>[4x]MFPDGFVWGTSTAAYQIEGAVAEDGRTPSIWDTFSRTKGKVVNGDTGDVACDHYHRWEEDLDLLAELGVQAYRFSVAWPRIHPDVTGPANQ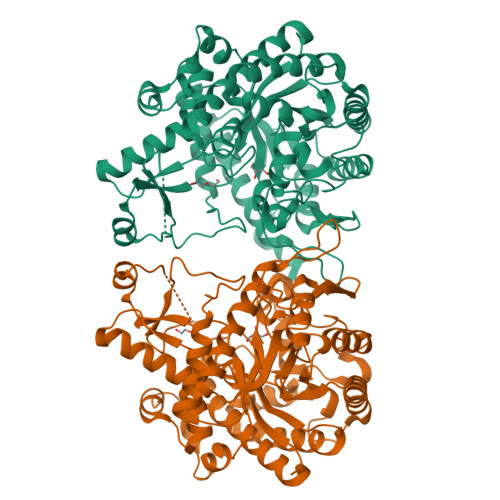KGLDFYQRLIDGLRDRNIIPLPTMYHWDLPQALEDEGGWIVRDTALRFADYAATVLEKLDGIDKWTTFNEPWTSAWLGYGYGHHAPGRTDIGAAAAATHHLLLAHGLGVQAARAIRPHVEIGLTLNLGVLRPGTTEDQDVEATWRADGNQNRIWLDPLFKGEYPADMIEHYSRWTPGFHTVQNGDLEIISSPIDFLGVNFYGPGTVMNVGREDAARAAGFNVGPRPESDEDNHLRCIGVETPGRPKTAMGWEVDATALRELLVRIKNEYTDIPLYITENGAAYHDYVNASGDVKDPERITYLNDHLEACLGAIDDGVNLQGYFIWSLLDNFEWGFGYSRRFGIVWIDYDTGRRIPKASYRWYQGVVATNGLPDLDGHLDTLN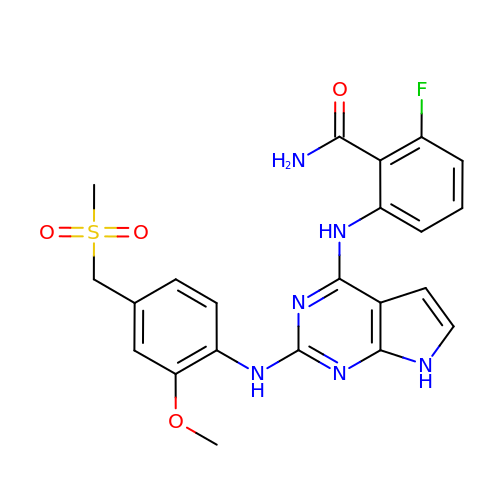2-fluoro-6-{[2-({2-methoxy-4-[(methylsulfonyl)methyl]phenyl}amino)-7H-pyrrolo[2,3-d]pyrimidin-4-yl]amino}benzamide | C22 H21 F N6 O4 S | VGYXXQRDIVRILX-UHFFFAOYSA-N>[4x]MNLKDKI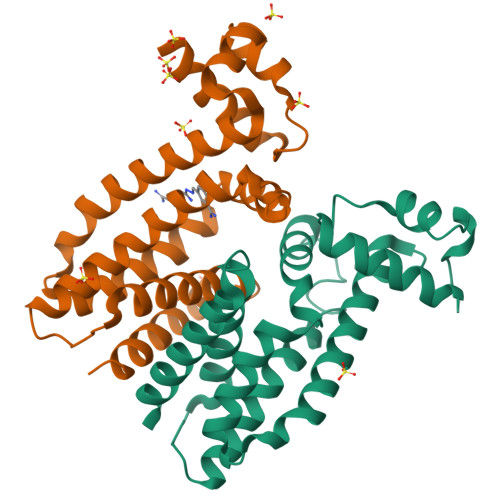LGVAKELFIKNGYNATTTGEIVKLSESSKGNLYYHFKTKENLFLEILNIEESKWQEQWKKEQIKAKTNREKFYLYNELSLTTEYYYPLQNAIIEFYTEYYKTNSINEKMNKLENKYIDAYHVIFKEGNLNGEWSINDVNAVSKIAANAVNGIVTFTHEQNINERIKLMNKFSQIFLNGLSK4-chloranyl-~{N}-[2-(piperidin-1-ylmethyl)-3~{H}-benzimidazol-5-yl]benzamide 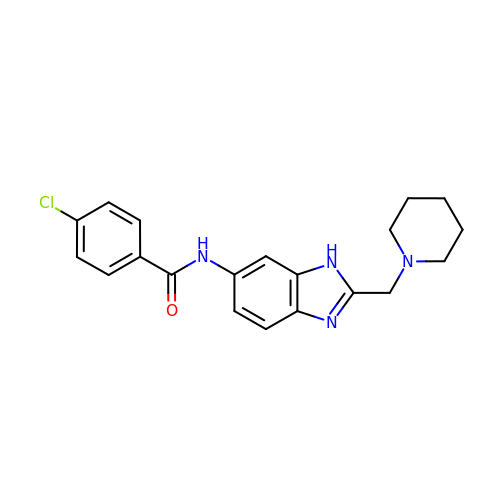| C20 H21 Cl N4 O | BKSMGCKPKGVUHS-UHFFFAOYSA-N>[4x]MLKFRTVHGGLRLLGIRRTSTAPAASPNVRRLEYKPIKKVMVANRGEIAIRVFRACTELGIRTVAI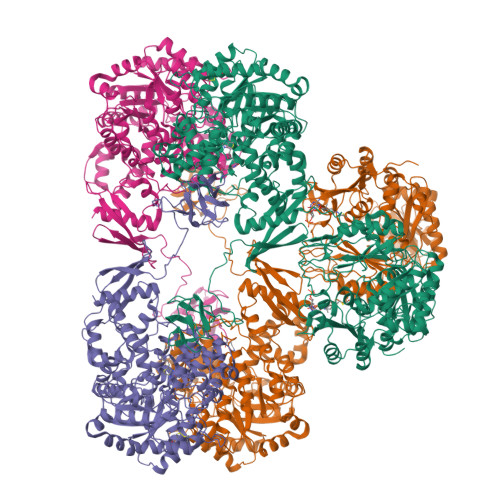YSEQDTGQMHRQKADEAYLIGRGLAPVQAYLHIPDIIKVAKENNVDAVHPGYGFLSERADFAQACQDAGVRFIGPSPEVVRKMGDKVEARAIAIAAGVPVVPGTDAPITSLHEAHEFSNTYGFPIIFKAAYGGGGRGMRVVHSYEELEENYTRAYSEALAAFGNGALFVEKFIEKPRHIEVQILGDQYGNILHLYERDCSIQRRHQKVVEIAPAAHLDPQLRTRLTSDSVKLAKQVGYENAGTVEFLVDRHGKHYFIEVNSRLQVEHTVTEEITDVDLVHAQIHVAEGRSLPDLGLRQENIRINGCAIQCRVTTEDPARSFQPDTGRIEVFRSGEGMGIRLDNASAFQGAVISPHYDSLLVKVIAHGKDHPTAATKMSRALAEFRVRGVKTNIAFLQNVLNNQQFLAGTVDTQFIDENPELFQLRPAQNRAQKLLHYLGHVMVNGPTTPIPVKASPSPTDPVVPAVPIGPPPAGFRDILLREGPEGFARAVRNHPGLLLMDTTFRDAHQSLLATRVRTHDLKKIAPYVAHNFSKLFSMENWGGATFDVAMRFLYECPWRRLQELRELIPNIPFQMLLRGANAVGYTNYPDNVVFKFCEVAKENGMDVFRVFDSLNYLPNMLLGMEAAGSAGGVVEAAISYTGDVADPSRTKYSLQYYMGLAEELVRAGTHILCIKDMAGLLKPTACTMLVSSLRDRFPDLPLHIHTHDTSGAGVAAMLACAQAGADVVDVAADSMSGMTSQPSMGALVACTRGTPLDTEVPMERVFDYSEYWEGARGLYAAFDCTATMKSGNSDVYENEIPGGQYTNLHFQAHSMGLGSKFKEVKKAYVEANQMLGDLIKVTPSSKIVGDLAQFMVQNGLSRAEAEAQAEELSFPRSVVEFLQGYIGVPHGGFPEPFRSKVLKDLPRVEGRPGASLPPLDLQALEKELVDRHGEEVTPEDVLSAAMYPDVFAHFKDFTATFGPLDSLNTRLFLQGPKIAEEFEVELERGKTLHIKALAVSDLNRAGQRQVFFELNGQLRSILVKDTQAMKEMHFHPKALKDVKGQIGAPMPGKVIDIKVVAGAKVAKGQPLCVLSAMKMETVVTSPMEGTVRKVHVTKDMTLEGDDLILEIE> MEFKDFPLKPEILEALHGRGLTTPTPIQAAALPLALEGKDLIGQARTGTGKTLAFALPIAERLAP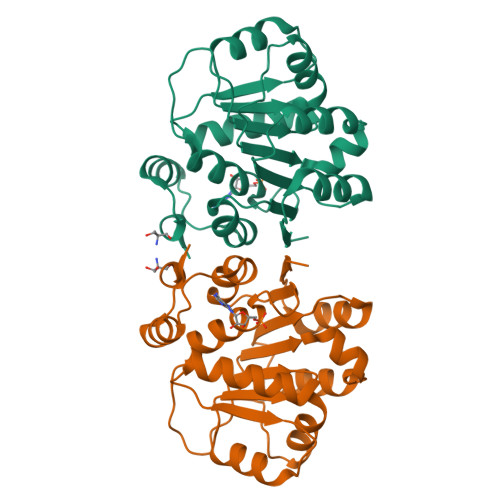SQERGRKPRALVLTPTRELALQVASELTAVAPHLKVVAVYGGTGYGKQKEALLRGADAVVATPGRALDYLRQGVLDLSRVEVAVLDEADEMLSMGFEEEVEALLSATPPSRQTLLFSATLPSWAKRLAERYMKNPVLINVIK> GAMAKKLSRTISGVTPVAVMTKPLPCPGKCIYCPTFAATPQSYTPESPAVLRAKSCEYQAYKQVALRLRIIQDMGHPTDKVELIIMGGTFLSADITYQYGFIKDCYDALNGVVAGSLEEAKTINETAQHRCVGLCIETRPDICGKAEIQRMIDFGTTRVELGVQMLDDDIYKLVERGHRVSDVAEATCLLREYGLKVH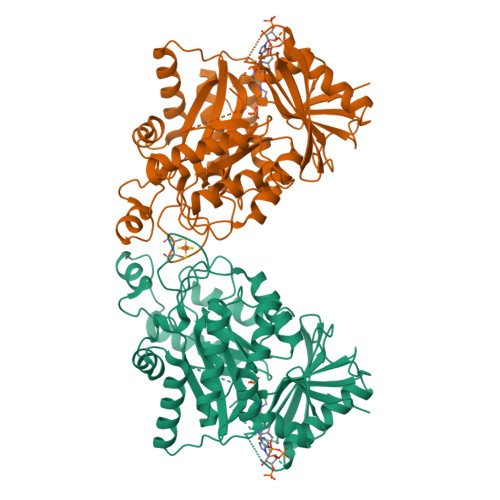YHWMPGLPGSSPEKDLALSRMVFEDPRFCPDGLKLYPTMVVEGTILEQWWKEGRYTPYPNGTMTGLIADIKALVPPYVRISRVLRDIPAVFISAGLKDSLRDGVRQILESRHQKCRCIRCREYGHRQRKGQTSGEPTLRRLDYPASGGKEIFLSFEDASDTLYGLLRLRIPCASLPVLGQKYGAKTGLVRALHVGSGSGRGLGRKLLAEAECLARDEFGLDSLAILSGVGAREYYRSLGYELVAGYMCKHLD Here we use deep network hallucination to generate a wide range of symmetric protein homo-oligomers given only a specification of the number of protomers and the protomer length. Starting from only a choice of chain length L and oligomer valency N (2 for a dimer, 3 for a trimer, etc.), the method carries out a Monte Carlo search in sequence space starting from a random sequence. The loss function guiding the search is computed by inputting N copies of the sequence into the AlphaFold2 (AF2) network, and combining structure prediction confidence metrics (pLDDT; per-residue structural accuracy, and pTM; an estimate of the TM-score) with a measure of cyclic symmetry (the standard deviation of the distances between the center of mass of adjacent protomers within the predicted structure). To eliminate such over-fitting, we generated new sequences for the HAL backbones using the recently developed ProteinMPNN sequence design neural network (accompanying manuscript: Dauparas et al.).

To evaluate design accuracy we attempted crystallization of 19 designs and succeeded in solving crystal structures for seven (three C2s, two C3s and two C4s). All crystal structures had the correct oligomerization state and closely matched the design models (median Cα RMSD of 0.6 Å across all designs, with resolutions ranging from 1.8 to 3.4 Å). The side chain conformations in the crystal structures also closely match those of the design models. HALC3_109 is a homo-trimeric three-layer all-helical structure, with three inner helices splaying outwards to contact two additional helices from the same protomers at angles of roughly 25° and 90°; the closest assembly in the PDB has a TM-score of 0.69.

>[6x]MSGREEIEEAVKEAELKVLAIVLVALRSVSHYEPLSRLYESFLDALKKALSEEELKEVEKEAERIEKKGS>[8x]ATMTLTDANFQQAIQGDKPVLVDFWAAWCGPCRMMAPVLEEFAEAHADKVTVA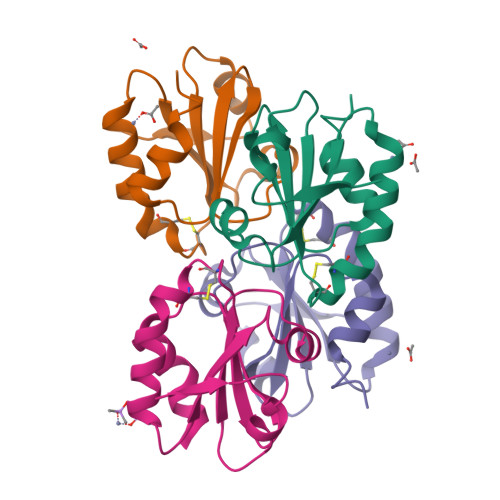KLNVDENPETTSQFGIMSIPTLILFKGGEPVKQLIGYQPKEQLEAQLADVLQ> TQAKAKHADVPVNLYRPNAPFIGKVISNEPLVKEGGIGIVQHIKFDLTGGNLKYIEGQSIGIIPPGVDKNGKPEKLRLYSIASTRHGDDVDDKTISLCVRQLEYKHPESGETVYGVCSTYLTHIEPGSEVKITGPVGKKMLLPDDPEANVIMLATGTGIAPMRTYLWRMFKDAERAANPEYQFKGFSWLVFGVPTTPNILYKEELEEIQQKYPDNFRLTYAISREQKNPQGGRMYIQDRVAEHADQLWQLIKNQKT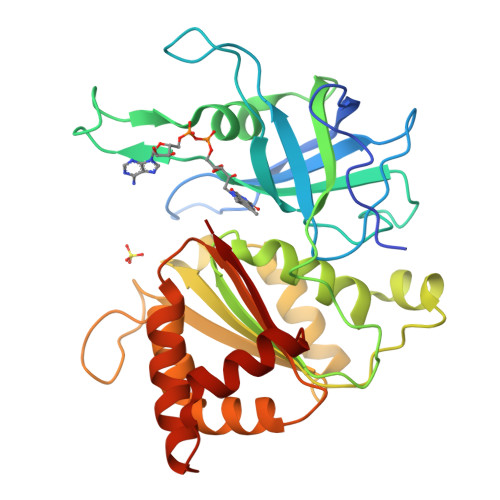HTYICGLRGMEEGIDAALSAAAAKEGVTWSDYQKDLKKAGRWHVETY>[3x]MENKGTNLTPEQALDRLEELYEQSVNALREAIADYVDNGTLPDPHARLNGLFVYPSLSVSWDGATPNPPKTRAFGRFTHPGCYTTTVTRPALFRAYLLEQLNLVYHDYGAHIAVEASHHEIPYPYVIDGSALTLDRSMSAGLTRHFPTTELAQIGDETADGLFHPGEFYPLSHFDARRVDFSLARLRHYTGTPVEHFQPFVLFTNYTRYVDE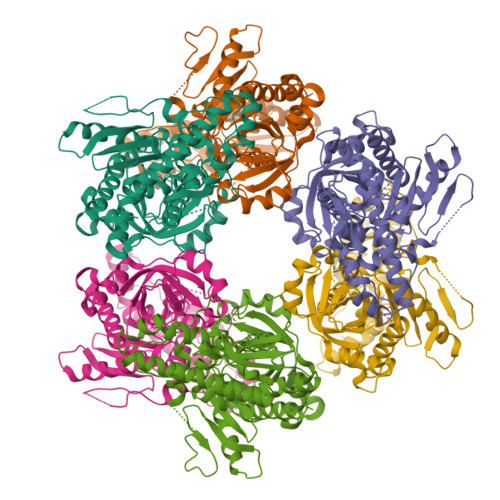FVRWGCSQILDPDSPYIALSCAGGIWITAETEAPEEAISDLAWKKHQMPAWHLVTADGQGITLVNIGVGPSNAKTICDHLAVLRPDVWLMIGHCGGLRESQAIGDYVLAHAYLRDDHVLDAVLPPDIPIPSIAEVQRALYDATKAVSGMPGEEVKQRLRTGTVVTTDDRNWELRYSASALRFNLSRAVAIDMESATIAAQGYRFRVPYGTLLCVSDKPLHGEIKLPGQANRFYEGAISEHLQIGIRAIDLLRAEGDRLHSRKLRTFNEPPFR> SDTAPAGFQLERVVILSRHGVRAPTKMTQTMRDVTPHQWPEWPVKLGYITPRGE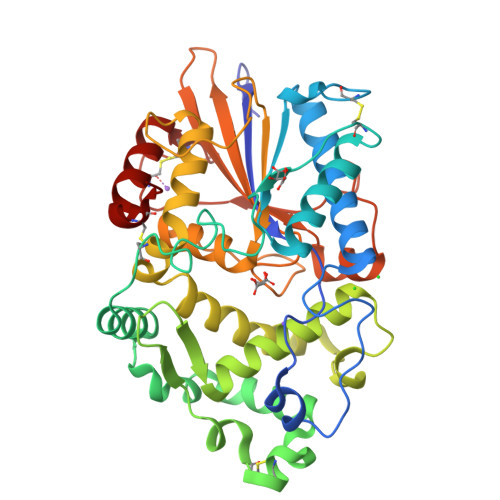HLISLMGGFYRERFQQQGLLPKDNCPTPDAVYVWADVDQRTRKTGEAFLAGLAPQCDLAIHHQQNTQQADPLFHPVKAGICSMDKSQVHAAVEKQAGTPIETLNQRYQASLALMSSVLDFPKSPYCQQHNIGKLCDFSQAMPSRLAINDDGNKVALEGAVGLASTLAEIFLLEHAQGMPKVAWGNIHTEQQWNSLLKLHNAQFDLMSRTPYIAKHNGTPLLQTIAHALGSNITSRPLPDISPDNKILFIAGHDTNIANISGMLGMTWTLPGQPDNTPPGGALVFERWVDNAGKPYVSVNMVYQTLAQLHDQAPLTLQHPAGSVRLNIPGCSDQTPDGYCPLSTFSRLVSHSVEPACQLP> SNINEREKERVALNKTAHSQGIEGKAMSEEWARYYPRQFDSWKKTKESDNITDMLKEKPALVVAWAGYPFSKDYNAPRGHYYALQDNINTLRTGAPVDGKTGPLPSACWTCKSPDVPRIIEQDGELEYFTGKWAKYGDEIVNTIGCYNCHDDKSAELKSKVPYLDRGLSAAGFKTFAESTHQEKRSLVCAQCHVEFYFKKTEWKDDKGVDKTAMVVTLPWSKGISTEQMEAYYDEINFADWTHGISKTPMLKAQHPDWELYKTGIHGQKGVSCADCHMPYTQEGAVKYSDH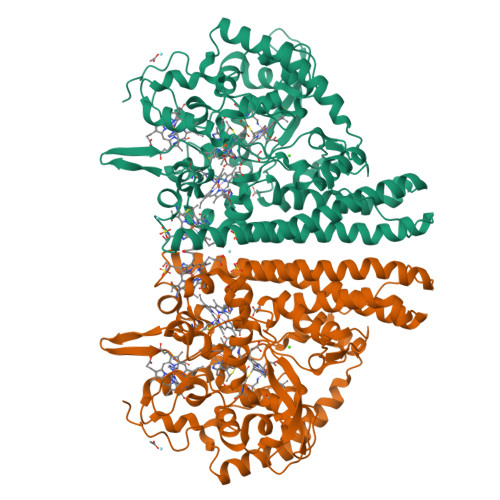KVGNPLDNMDKSCMNCHRESEQKLKDIVKQKFERKEFLQDIAFDNIGKAHLETGKAMELGATDAELKEIRTHIRHAQWRADMAIAGHGSFFHAPEEVLRLLASGNEEAQKARIKLVKVLAKYGAIDYVAPDFETKEKAQKLAKVDMEAFIAEKLKFKQTLEQEWKKQAIAKGRLNPESLKGVDEKSSYYDKTKK> GEDRRVPQNWFPIFNPERSDKPNASDPSVPLKIPLQRNVIPSVTRVLQQTMTKQQVFLLERWKQRMILELGED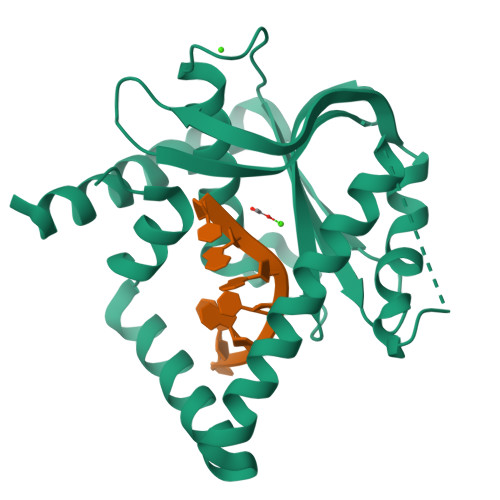GFKEYTSNVFLQGKRFQEALESILSPQETLKERDENLLKSGYIESVQHILKDVSGVRALESAVQHETLNYIGLLDCVAEYQGKLCVIDWKTSEKPKPFIQSTFDNPLQVVAYMGAMNHDTNYSFQVQCGLIVVAYKDGSPAHPHFMDAELCSQYWTKWLLRLEEYTEKKKNQNIQKPEYSE> MTEHFITLSTTEPNNNIGIVKLRHADVNSQAIVAQIVENGQPKNFEGLQPFFCLMAQEATGQGVSEESVVSFDAKNGTLKYVASDNALQFVGRNEAYFSFRKQEGG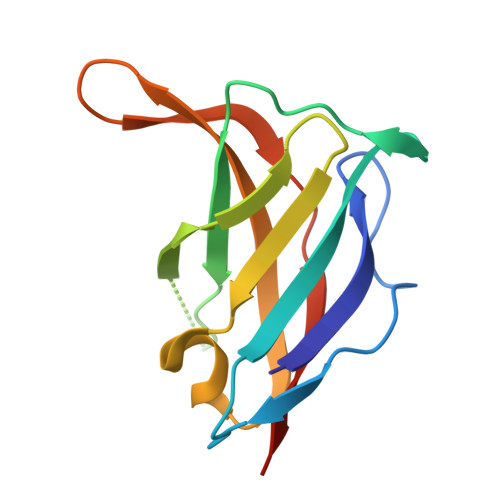RWIEQFSTRTFHYIVEKSIYSQ> DAMNREVSSLKN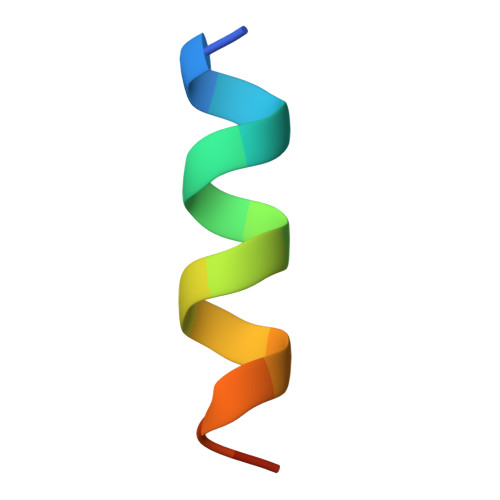KLRR> GSEFSAMMYIQELRSGLRDMHLLSCLESLRVSLNNNPVSWVQTFGAEGLASLLDILKRLHDEKEETSGNYDSRNQHEIIRCLKAFMNNKFGIKTMLETEEGILLLVRAMDPAVPNMMIDAAKLLSALCILPQPEDMNERVLEAMTERAEMDEVERFQPLLDGLKSGTSIALK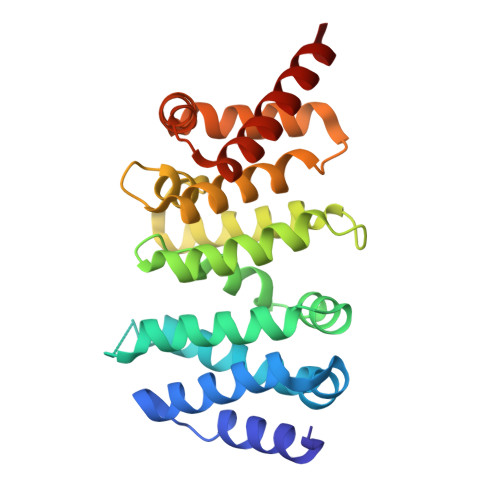VGCLQLINALITPAEELDFRVHIRSELMRLGLHQVLQELREIENEDMKVQLCVFDEQGDEDFFDLKG> MPFQQGLLATPVPAHARHLFFTLQSPEALPAALDALLPQVDGKQLLLGVGAPLAKALGREIPGLRPFPLLDAAVENPSTQHALWLWLRGDERGDLLLRTQALEQALAPALSLADSVDGFLHRGGYDLTGYEDGTENPTDEEVVQAAIAADGSSFAAFQLWKHDLQYFKSLPQADQDNIIGRRLSDNEKLDDAPASAHVKRTA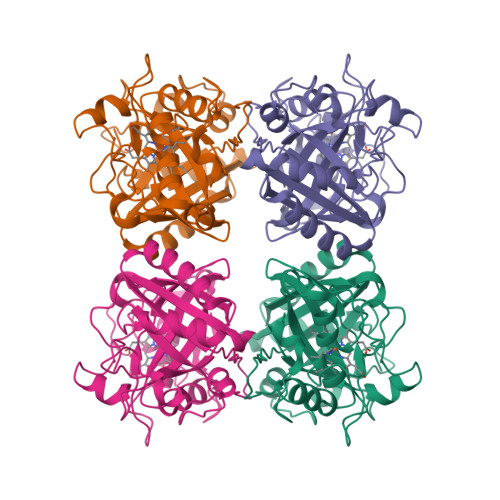QESFEPEAFMVRRSVSWADQRGAGLAFVALGKSFEAFEVQLRRMSGLEDGIIDGLYRFSRPLTGGYYWCPPMSETGVDLSPLLRA>[2x]GSYAEGQKKRRNTLHEFKKSAKTTLTKEDPLLKIKTKKVNSADECANRCIRNRGFTFTCKAFVFDKSRKRCYWYPFNSMSSGVKKGFGHEFDLYEN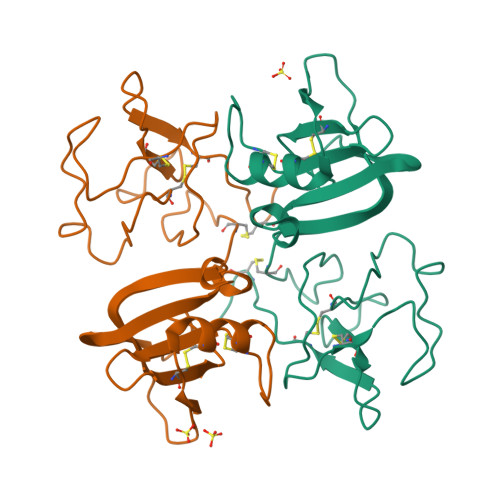KDYIRNCIIGKGGSYKGTVSITKSGIKCQPWNSMIPHEHSFLPSSYRGKDLQENYCRNPRGEEGGPWCFTSNPEVRYEVCDIPQCSEV> 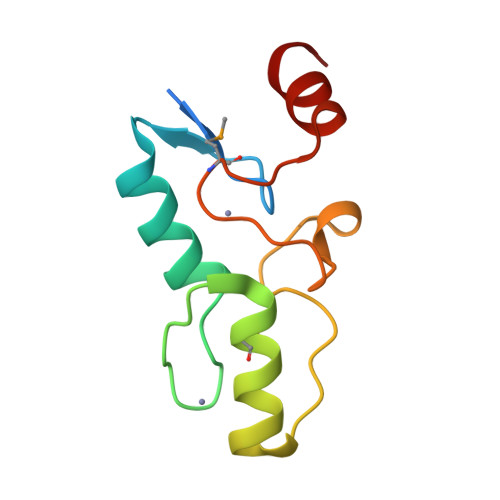MGKKKKRVEKVFCYYCDREFDDEKILVQHQKAKHFKCHVCHKKLSTAGGMAIHVLQVHKESVTKVPNAKPERESTEIEIFGMQGIPPDVLAAHYGE> MSLKLISNDLRDGDKLPHRHVFNGMGYDGDNISPHLAWDDVPAGTKSFVVTCYDPDAPTGSGWWHWVVVNLPADTRVLPQGFGSGLVAMPDGVLQTRTDFGKTGYDGAAPPKGETHRYIFTVHALDIERIDVDEGASGAMV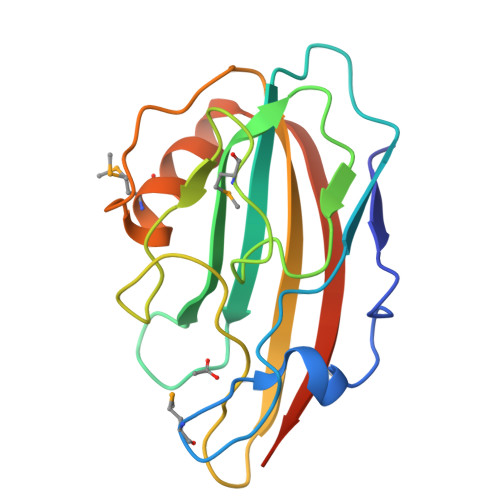GFNVHFHSLASASITAMFSEGGSHHHHHH> MGHHHHHAYTLSKSGKEKEEVDEILEEEAEVDELKSPESVVQLLHIDPIEFEFGYGLIPLADANQGGDLLDRIVMIRRQLALELGLVIPVVRIRDNIALQPNEYRLKIKGNEVAKGELLLDHYLAMSPTPEDDLIEGIETVEPSFGLPAKWISEAVKDEADMLGYTVVDPASVVSTHITEKIKQHAHEL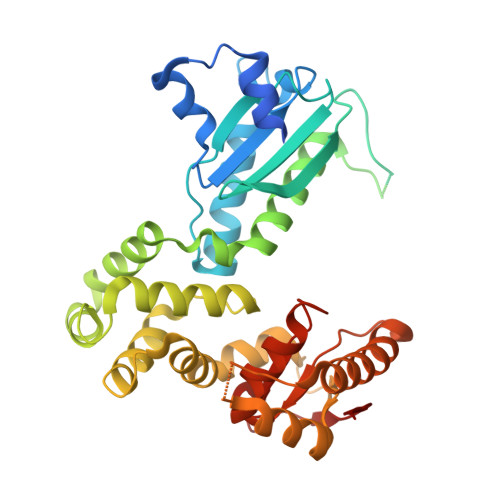IGRQETKQLIDHLKESYPVLVEEVTPNPLSVGDIQKVLAKLLKEKVSIRNLVTIFETLADYGKLTTDSDLLTEYTRQALAKQITAQFAKENEVLKVVTCSGRVEKAIADGVQQTEHGNYLSLEPDISESIVRSVAKEAEQLSLRQETAILLCSPPVRMYVKQLLERYFPDLPVLSYNELEANVEVQSIGVVDI> LSNEDPKDALLRQFQKEIEELKKKLEELEKERDFYFGKLRNIELICQENEGENDPVLQRIVDILYATDEGFVIP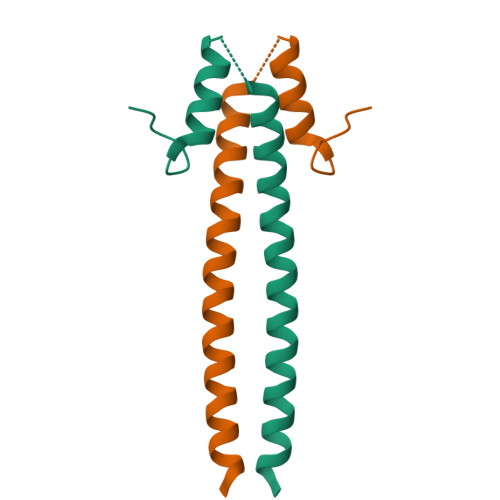D>[4x]MEAVPRMPMIWLDLKEAGDFHFQPAVKKFVLKNYGENPEAYNEELKKLELLRQNAVRVPRDFEGCSVLRKYLGQLHYLQSRVPMGSGQEAAVPVTWTEIFSGKSVAHEDIKYEQACILYNLGALHSML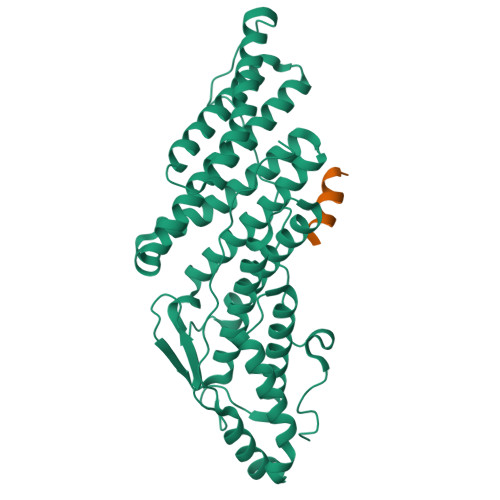GAMDKRVSEEGMKVSCTHFQCAAGAFAYLREHFPQAYSVDMSRQILTLNVNLMLGQAQECLLEKSMLDNRKSFLVARISAQVVDYYKEACRALENPDTASLLGRIQKDWKKLVQMKIYYFAAVAHLHMGKQAEEQQKFGERVAYFQSALDKLNEAIKLAKGQPDTVQDALRFTMDVIGGKYNSAKKDNDFIYHEAVPALDTLQPVKGAPLVKPLPVNPTDPAVTGPDIFAKLV;>QRAEEEDDDIKQLAAWAT[4x]> MTNIVGRIGFLTTGKLGIKLRGVLIDESTTPNTTYLPGIESFFNITANVLTSVSYPETETQNVTATFSIYSVDGSSNPVFPALLSFDAIVPN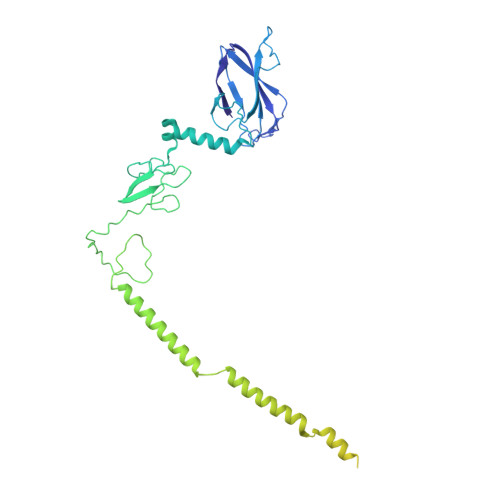VASVEFDVLAPTGVVNNQLDTSALRIAKIIANDPALAQKVAGAPYPRGAYSATETYLYGEMVSYFGKNYISKSLSPIINILPTVTDSWYELVITLPESVSVIATGSDTAYGTGWNGSLLVPTQNAVYDKIVTVDAAIATANTNITNLGTAKADLSYVNTQLSADQVVLDALSSGKADLSYVNTQLNSKANLNGAVLVNATTATPPISDNDTSLATTQHVRSFNHSRLAFNAFRGGQQGVPSLSYVTTTAQFNSSSVRSGWGDNFSSNRWLVGEGGTYLITVTTRFATVGGTPPTYFDALLFVGLSGSGVENFLTRSQSVYPSFGYTLSWVGILTFNTGQNVFLNYQVNAVGGGSYSVVLEDVRFSGIQLG>GSHMTHRVALITGGSRGIGAAIALKLAQDGFDIAITYARNEKAAQKVVSEVEALGRKAVAVQADGGSTDGNIAAITKTHEAFGRLDALVCNAGIYPYGPIAQMTVTQIEEVLNLNLRAAMVETVEALKYMKTGGRLIYIGSAFGERAPFPGISLYAATKAGLIGFTKGVARDLGPQGITA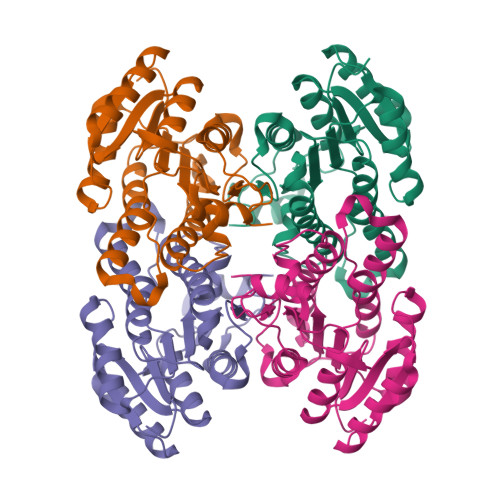NVVEPGPIATDLNPEDGAAAAVIRKFTATESYGKVNDIARTVSFLASPDASYITGASILVDGGLVA[8x]The soluble ACh-binding proteins (AChBP) from mollusks form homopentameric assemblies of subunits homologous to the N-terminal, extracellular ligand binding domain (LBD) of the nAChR (Figure A1). The binding pocket of AChBP possesses all of the functional residues identified in the nAChR LBD, and its extension toward various directions of the interface provides multiple means for selective accommodation of the nicotinic ligands. The ligand binding pocket encompasses a nest of five electron-rich aromatic side chains provided by residues Tyr93, Trp147, Tyr188 and Tyr195 on the principal (+) face of the subunit interface and residue Tyr55 on the complementary (−) face. This pocket is partially sheltered from the solvent by loop C, which is found at the outer perimeter of the pentamer and harbors at its tip a disulfide bridge linking the vicinal Cys190 and Cys191 residues, linked into a Cys-trans-Cys disulfide bridge (aka oxidized cysteinyl-cysteinyl ring), a signature determinant for nAChR α subunits.

Initial electrophysiology experiments on nAChRs and binding and crystallography experiments on AChBPs were carried out using the racemic spiroimine (±)-4. Co-crystallization of A-AChBP with the (±)-4 racemate unambiguously led to a bound (+)-4 R enantiomer at all five subunit interfaces in a virtually identical position to that seen in the (+)-4 R complex, with only a minor trace (i.e., occupancy below ~10%) of a bound (−)-4 S. Per se, this observation would suggest a much lower dissociation rate for enantiomer (+)-4 R relative to its (−)-4 S congener than the one recorded through the binding studies. Whether this is due to the more acidic and hydrophobic composition of the crystallization liquor used for the (±)-4 complex compared with the other two complexes or to conformational remodeling of the complex during crystal nucleation and growth is unknown. Overall, the DX scoring approach appears consistent with the prevailing presence of enantiomer (+)-4 R in the structure of the complex prepared from the (±)-4 racemate. In all three complexes, the loop-C position shows a high degree of variability with respect to the different orientation of the 3-ring system in each enantiomer associated with slightly different orientations of the bound enantiomers at each binding interface. In the (±)-4 and (−)-4 S complexes, loop C clusters around intermediate positions in all five subunits. However, the loop-C “intermediate” positions associated with its loose interactions with the spiroimines resemble more the position observed in HEPES-bound or apo AChBPs than that in complexes with small agonists.

>[5x]DYKDDDDKLHSQANLMRLKSDLFNRSPMYPGPTKDDPLTVTLGFTLQDIVKADSSTNEVDLVYYEQQRWKLNSLMWDPNEYGNITDFRTSAADIWTPDITAYSSTRPVQVLSPQIAVVTHDGSVMFIPAQRLSFMCDPTGVDSEEGATCAVKFGSWVYSGFEIDLKTDTDQVDLSSYYASSKYEILSATQTRQVQHYSCCPEPYIDVNLVVKFRERR>[2x]ANPCCSNPCQNRGECMSTGFDQYKCDCTRTGFYGENCTTPEFLTRIKLLLKPTPNTVHYILTHFKGVWNIVNNIPFLRSLIMKYVLTSRSYLIDSPPTYNVHYGYKSWEAFSNLSYYTRALPPVADDCPTPMGVKGNKELPDSKEVLEKVLLRREFIPDPQGSNMMFAFFAQHFTHQFFKTDHKRGPGFTRGLGHGVDLNHIYGETLDRQHKLRLFKDGKLKYQVIGGEVYPPTVK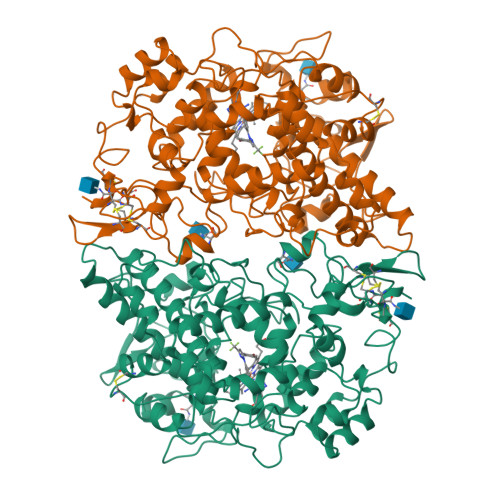DTQVEMIYPPHIPENLQFAVGQEVFGLVPGLMMYATIWLREHQRVCDILKQEHPEWGDEQLFQTSKLILIGETIKIVIEDYVQHLSGYHFKLKFDPELLFNQQFQYQNRIASEFNTLYHWHPLLPDTFNIEDQEYSFKQFLYNNSILLEHGLTQFVESFTRQIAGRVAGGRNVPIAVQAVAKASIDQSREMKYQSLNEYRKRFSLKPYTSFEELTGEKEMAAELKALYSDIDVMELYPALLVEKPRPDAIFGETMVELGAPFSLKGLMGNPICSPQYWKPSTFGGEVGFKIINTASIQSLICNNVKGCPFTSFNVQDPQPTKTATINASASHSRLDDINPTVLIKRRSTEL The N-terminal (NT) domain of spider silk proteins (spidroins) is crucial for their storage at high concentrations and also regulates silk assembly. NTs from the major ampullate spidroin (MaSp) and the minor ampullate spidroin are monomeric at neutral pH and confer solubility to spidroins, whereas at lower pH, they dimerize to interconnect spidroins in a fiber. Here, we determine the solution and crystal structures of the flagelliform spidroin NT, which shares only 35% identity with MaSp NT, and investigate the mechanisms of its dimerization. However, the protonation events involve a different set of residues than in MaSp, indicating that an overall mechanism of pH-dependent dimerization is conserved but can be mediated by different pathways in different silk types.

The X-ray crystal structure of FlSp NT dimer was also solved and contained a single dimer in crystallographic asymmetric unit. The model could be built for most of the protein, excluding NT residues 1 to 9 in subunit A and 1 to 11 in subunit B, C-terminal residue of subunit A and loop, including residues 55 to 59 of subunit A. All the obtained structures were compared to WT MaSp NT in order to determine the overall structural similarity and to identify structural differences for the key residues. The high-resolution X-ray structure reveals more details on pH-dependent interactions between acidic residues of monomers. The most obvious such interaction occurs among Asp 122 and Glu 130 of both subunits. This interaction is possible only at low pH and requires that at least one of the acidic residues—presumably Glu 130—is protonated. Another notable contact occurs among Glu 84 and Asp 41 of the same subunit, described previously as “handshake interaction” in MaSp NT. This interaction in turn may alter the relative placement of α-helices and favor necessary interactions between monomers, such as salt bridge formation among Glu 40 and Arg 59 of the other subunit. However, this salt bridge is present only in one side of the dimer, since the loop, including Arg 59 is disordered in the other monomer of our crystal structure. The intersubunit salt bridge formed between Asp 40 and Lys 65 in MaSp NT is also present between Asp 41 and Lys 65 in FlSp NT and an additional interaction between Asp 44 and Lys 65 was identified. Based on the X-ray structure of FlSp NT, Glu 130 was identified as a promising candidate as its protonation would favor dimer formation by alleviating the electrostatic repulsions with negatively charged residues present at the dimer interface, and this supposition agrees with major chemical shift changes of Gln 131 upon dimerization of FlSp NT.

>[2x]GSGNSASQSPFSNPNTAEAFARSFVSNIVSSGEFGAQGAEDFDDIIQSLIQAQSMGKGRHDTKAKAKAMQVALASSIAELVIAESSGGDVQRKTNVISNALRNALMSTTGSPNEEFVHEVQDLIQMLSQEQINEV In this study, by means of glycan microarray screening, NMR, surface plasmon resonance (SPR), and cell binding assays, we show that FA, which is the predominant glycolipid in ovine erythrocytes, serves as a cellular attachment receptor for the VP1 of a polyomavirus originally identified in sheep. This designated sheep polyomavirus (ShPyV) is a member of a non-enveloped, double-stranded DNA virus family with icosahedral capsids, scaffolded by the major capsid protein VP1. Here, glycan array screening shows that the major capsid protein VP1 of sheep polyomavirus (ShPyV) binds to the Forssman glycolipid, an antigen of many vertebrates and a potential tumor marker in humans. We show that the Forssman antigen serves as a cellular attachment receptor for the major capsid protein VP1 of ShPyV. Thus, our studies present the first example of a polyomavirus VP1 protein interacting with a non-sialyl neutral glycan, complementing the principles of how polyomaviruses recognize their targets.

To characterize the binding of Forssman antigen by ShPyV VP1 with atomic detail, we solved the crystal structure of the VP1 in complex with 10 mM of Forssman pentaose (F_P_) at 1.92 Å resolution. All five Forssman binding sites are identical and located between two neighboring VP1 monomers ([Fig fig4]). In the binding sites without artificial crystal contacts, electron density provides an unambiguous outline of the last four monosaccharides of F_P_ ([Fig fig4]). The intermolecular contacts show that the terminal trisaccharide of F_P_ contributes to binding, whereas the remaining βGal and Glc divert away from VP1 and do not interact with the protein surface. Closer inspection of the binding site reveals that the methyl group of the terminal αGalNAc invades a hydrophobic surface depression constituted by phenylalanine residues of two neighboring VP1 monomers, establishing van der Waals interactions ([Fig fig4]). Additionally, the *N*-acetyl moiety of αGalNAc interacts with the Q266 and F66cw residues via hydrogen bonds ([Fig fig4]). In βGalNAc, the carbonyl oxygen forms two hydrogen bonds with the side chains of Q266 and N268 ([Fig fig4]). Apart from these contacts, numerous interactions involve the hydroxyl groups of F_P_ that are directed towards the protein surface. By the assessment of our ShPyV VP1-Forssman pentaose (F_P_) complex structure, the designated minimal glycan binding motif is the GalNAcα1-3GalNAc disaccharide with few additional contacts to the subsequent αGal. From structural perspective, this epitope recognition clearly disallows branching of the glycan at certain positions, e.g., O3 of αGalNAc, N2 of βGalNAc or O4 of αGal.

>[10x]GSHMGGIEVLAVRTGPDSITEIEAYLNPRMGQPQNEDFYGFSDNVTVSDDFGSDAPPWKQFPCYSTARISLPMLNQDMTSDTILMWEAISCRTEVMGVNMLTNVHSAQKRVYENDREGTGIGVEGMGYHMFAIGGEPLELQFMVFNHRATYPAEATVIKNPGASSQVFDPNLKGTLTADGVFPVEAWGPDPFKNENTRYFGQYTGGTQTPPVLTFTNTQTTILLDENGVGPLCKGDGLFLSCADIVGFFTQHNKKMSFRGLPRYFRVTLRKRVVKN> RNGKSQ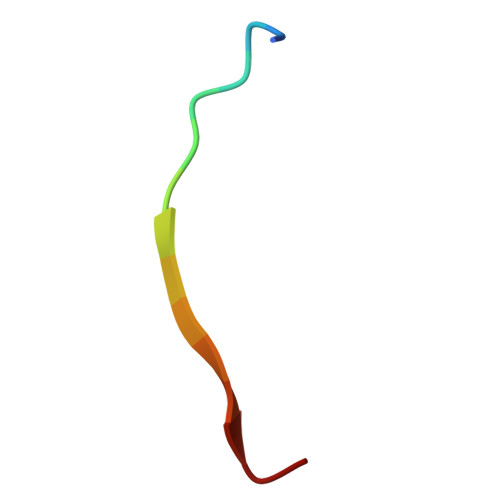SIIVGPWGD> GPLGSRLEQYEIHI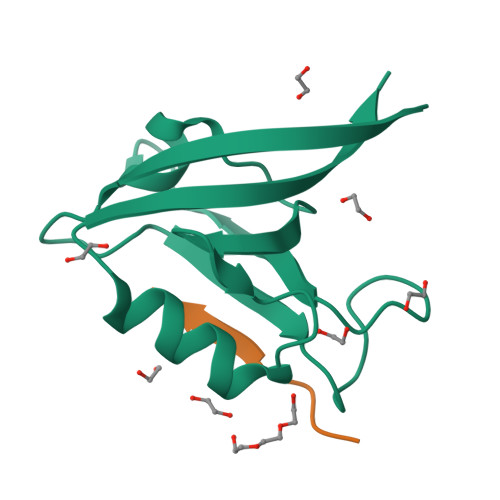ERTAAGLGLSIAGGKGSTPFKGDDDGIFISRVTEAGPADLAGLKVGDKVIKVNGIVVVDADHYQAVQVLKACGAVLVLVVQREVTR;> LPSFETAL3-methyl-7-propyl-purine-2,6-dione | C9 H12 N4 O2 | 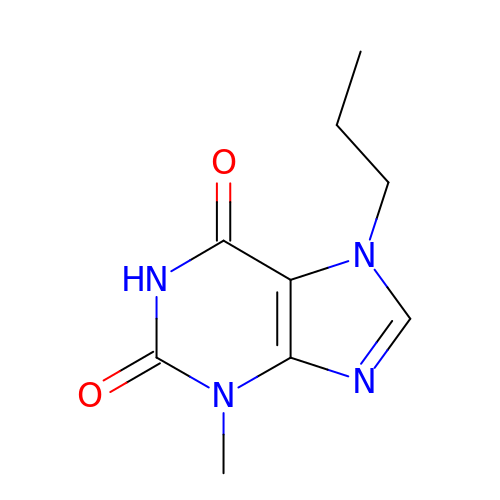MHNVSFOURBQRPK-UHFFFAOYSA-N>[2x]GPLGSESEDDKAFEENRRLR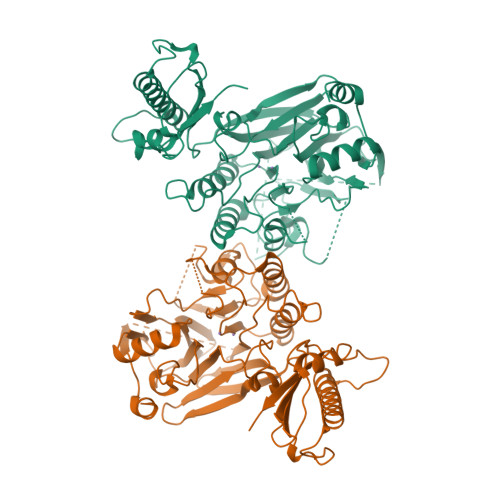NLGSVEYIRIMSSEKSNANSRHTSKYYSGRKNFKKFQKKASQKVDGSAGSAGSENTIRILISSDPHVGYGEKDPVRGNDSFVSFNEILEIARERDVDMILLGGDIFHDNKPSRKALYQALRSLRLNCLGDKPCELELLSDTSLTTGDTAVCNINYLDPNINVAIPVFSIHGNHDDPSGDGRYSALDILQVTGLVNYFGRVPENDNIVVSPILLQKGFTKLALYGISNVRDERLYHSFRENKVKFLRPDLYRDEWFNLLTVHQNHSAHTPTSYLPESFIQDFYDFVLWGHEHECLIDGSYNPTQKFTVVQPGSTIATSLSPGETAPKHCGILNITGKDFHLEKIRLRTVRPFIMKDIILSEVSSIPPMVENKKEVLTYLISKVEEAITEANAQWYEAQGTVPVVENEKPPLPLIRLRVDYTGGYQTENPQRFSNRFVGRVANATDVVQFYLKK>[2x]ETGELKIECPHTIGLGQGLVIGSVELPPVPLTQVESLKLESSCNFDLHTSTSSQQPFTKWTWEMKSDLAENTQASSTSFQTKSSEINLRGLCLVPPLVIETAARTRKTIACFDLSCNQTACQPTVFLIGPIQTCITTKSCLLGLGDQRIQVNYEKTYCVSGQLVEGVCFNPVHTMALSQPSHTYDIVTV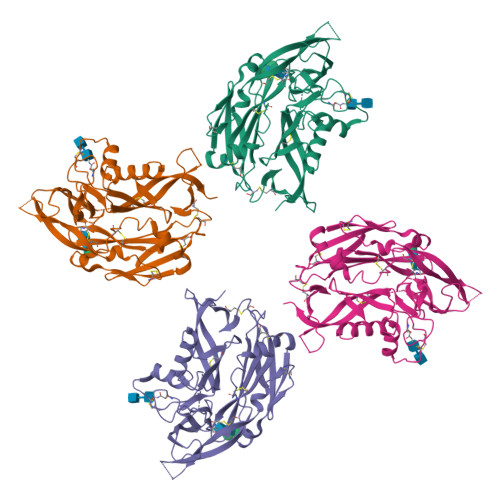MVRCFLIAKKVSTGDSMKLEKSFETLVQKTSCTGNGFQGYYICLVGSSSEPLYIPTLDDYRSAEVLSRMAFAPHGEDHDVEKNAISAMRIIGKVTGKAPSTESSDTIQGVAFSGNPLYTSTGVLTAKDDPVYIWAPGIIMEGNHSVCDKKTLPLTWTGFIPLPGEIEKT>[2x]MSYQDLKECKIITAFITPFHEDGSINFDAIPALIEHLLAHHTDGILLAGTTAESPTLTHDEELELFAAVQKVVNGRVPLIAGVGTNDTRDSIEFVKEVAEFGGFAAGLAIVPYYNKPSQEGMYQHFKAIADASDLPIIIYNIPGRVVVELTPETMLRLADHPNIIGVKECTSLANMAYLIEHKPEEFLIYTGEDGDAFHAMNLGADGVISVASHTNGD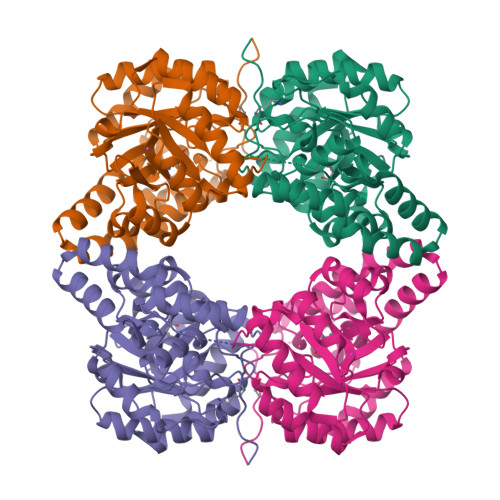EMHEMFTAIAESDMKKAAAIQRKFIPKVNALFSYPSPAPVKAILNYMGFEAGPTRLPLVPAPEEDVKRIIKVVVDGDYEATKATVTGVLRPDY>GGGIDYIKLLGEIATENQFEVTYVDIEEKTFSGQFQCLVQLSTLPVGVCHGSGPTAADAQRHAAQNALEYLKIMT[7x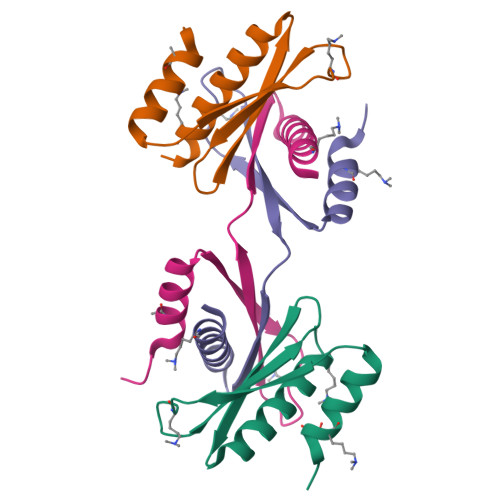];> AAAAAAAAAAAAAAAAAAAAAAAAAAAAAAAAAAAAAAAAAAAAAAAA> RPESELIRQSWRVVSRSPLEHGTVLFARLFALEPSLLPLFQYNGRQFSSPEDSLSSPEFLDHIRKVMLVIDAAVTNVEDLSSLEEYLTSLGRKHRAVGVRLSSWSTVGESLLYMLEKSLGPDFTPATRTAWSRLYGAVVQAMSRGWDG

To investigate the correlation between mechanical properties and functional efficiency in proteins, we selected neuroglobin (Ngb), a hexacoordinated heme protein, which is expressed in the neurons of vertebrates and is involved in neuroprotection in hypoxic conditions and protects brain from stroke. Ngb folds like all globins with a bundle of eight helices termed A to H, and a heme hexacoordinated in both ferric and ferrous forms by the imidazole side chain of the distal and proximal histidines (His 64 and His 96 respectively). The structures of human and murine Ngb present a large internal cavity behind the heme, that is connected to the surface through a tunnel, forming a pathway toward the heme for gaseous ligands (O2, CO, NO). Like many recently discovered globins, Ngb is characterized by endogenous heme iron hexacoordination in the absence of external ligands.

In the CO-Ngb structure, Phe 106 is the residue mostly affected by the shift of the heme inside the cavity. Its mutation to a Trp hampers heme displacement, leading to low CO affinity. The mutation of the Phe 106 to a Trp leads to a shift of the segment Lys 95 – Ser 107 (termed extended FG loop) toward the bulk. In particular, the side chain of Leu 103 is pushed towards the bulk by the side chain of Trp 106. The shift of Leu 103 leads to a shift of the side chain of Trp 148, located at the end of helix G, and to repositioning of the C-terminal Gly 150. Mean B-factors in the mutant are similar to the WT. The volume of the internal cavity is reduced by 4.6% upon the F to W mutation as expected.One such Rieske oxygenase is found in the organism Comamonas testosteroni, as part of the TsaMBCD pathway, which is involved in metabolizing 4-methylbenzenesulfonate and 4-methylbenzoate into protocatechuate. TsaC, an annotated short-chain dehydrogenase/reductase (SDR) enzyme, and TsaD, an annotated aldehyde dehydrogenase, are the next enzymes in the pathway. These proteins have been suggested to perform iterative NAD+-dependent oxidation reactions on the primary alcohol products of TsaM to produce 4-sulfobenzoate and 1,4-benzenedicarboxylate, respectively. Importantly, TsaC and TsaD also recycle the reducing equivalents used by TsaM and TsaB.

The crystal structure of TsaC was determined to a resolution of 2.18 Å using the structure of meso-2,3-butanediol dehydrogenase (BDH) as a model for molecular replacement. In the solved structure, there are two copies of TsaC in the asymmetric unit, each of which showcases a Rossmann fold and contains a central seven-stranded β-sheet and seven α-helices. Based on an approximate interface of 2837 Å2 (16.2% of the total monomeric surface area), these two subunits form a dimer, and like that observed in BDH, this dimer and two symmetry-related molecules assemble into a tetramer. Similar to the structure of BDH, and as described for other SDR enzymes that are considered classical members of the family, within the Rossmann fold, TsaC contains the expected sequence motifs for binding a nicotinamide coenzyme. However, decorating this binding site, and following β2, is residue Asp36. This residue is positioned similarly to other negatively charged residues in SDR enzymes that are credited with favoring the use of NAD(H). However, in both chains of TsaC, the hydroxyl and amino functional groups of the Tyr155 and Lys159 side chains are located approximately 10 Å apart and do not appear to be catalytically competent. This inactive conformation is a hallmark of other SDR enzymes that, like TsaC, do not have a nicotinamide coenzyme bound in the active site. In agreement with the observed inactive state of the catalytic tetrad, approximately 30 residues between β6 and α7 are too disordered to build and are therefore missing from both monomers in the refined structure of TsaC. The equivalent of the hinge residues in TsaC are Pro185 and Pro221, which bookend the unresolved loop.

>MGSSHHHHHHSSGENLYFQGMNLNKQVAIVTGGASGFGAAIARRLSQAGAAVLVADLNAEGAQRMATELNAAGGRALGMACDVSKEADYRAVVDAAIAQLGGLHIVVNNAGTTHRNKPALAVTEDEFDRVYRVNLKSVYWSAQCALPHFAQQGHGVMVNVASTTGVRPGPGLTWYSGSKAAMINLTKGLALEFARSGVRINAVNPMIGETPMMADFMGMEDTPANRERFLSRIPLGRFTRPDDVASAVAFLASDDASFLTGVCLDVDGGRNI[2x]>MTQELGNANFENFIGATEGFSEIAYQFTSHILTLGYAVMLAGLLYFILTIKNVDKKFQMSNILSAVVMVSAFLLLYAQAQNWTSSFTFNEEVGRYFLDPSGDLFNNGYRYLAWLIDVPMLLFQILFVVSLTTSKFSSVRNQFWFSGAMMIITGYIGQFYEVSNLTAFLVWGAISSAFFFHILWVMKKVINEGKEGISPAGQKILSNIWILFLISWTLYPGAYLMPYLTGVDGFLYSEDGVMARQLVYTIADVSSKVIYG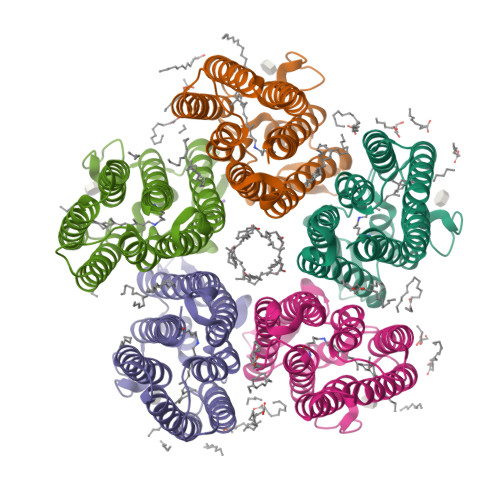VLLGNLAITLSKNKELVEANSLEHHHHHH[5x]> MAQTLQYVSSRLSMLQIDEEDLERNAQFGKVLIELCPLLGPNGGSANLNRELEETRRELLLQRKMWMRSEVIYQLVQEMLLDL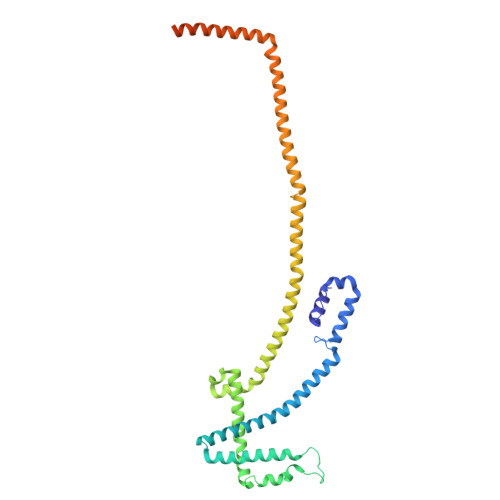QVRKLEGSLTEEERKFQDGLQQCMLVSECSRLLTADSVPPSDSTSILGLDKQDLLDLLPPNMLVLWVRDRLQKQLEEALKKKCFTFLSFHQPETDEEGDVLRAAKVLRLASTLEDEKRRLQNEQEKHQEMRALLEKQQEIYPHVLLRCLSLLRQAASELRLRAQSDIDRINAEYLEAKSNALFLKLRMEELQVLTDCYTPEKVLVHRQIRDTLEAGVKKEKQELSTSRQILSSYEFLGPEFEGLVQEYTRLKDKIKDNRWMLQELSKSLP> AAHHHHHHSSGLVPRGSHMANKAVNDFILAMNYDKKKLLTHQGESIENRFIKEGNQLPDEFVVIERKKRSLSTNTSDISVTATNDSRLYPGALLVVDETLLENNPTLLAVDRAPMTYSIDLPGLASSDSFLQVEDPSNSSVRGAVNDLLAKWHQDYGQVNNVPMQYEKITAHSMEQLKVKFGSDFEKTGNSLDIDFNSVHSGEKQIQIVNFKQIYYTVSVDAVKNPGDVFQDTVTVEDLKQRGISAERPLVYISSVAYGRQVYLKLETTSKSDEVEAAFEALIKGVKVAPQTEWKQILDNTEVKAVILGGDPSSGARVVTGKVDMVEDLIQEGSRFTADHPGLPISYTTSFLRDNVVATFQNSTDYVETKVTAYRNGDLLLDHSGAYVAQYYITWDELSYDHQGKEVLTPKAWDRNGQDLTAHFTTSIPLKGNVRNLSVKIRECTGLAWEWWRTVYEKTDLPLVRKRTISIWGTTLYPQVEDKVENAA

Gram-positive bacteria, including the common wound-infecting Staphylococcus aureus, the virulent food-borne pathogen Listeria monocytogenes, and Streptococcus pneumoniae that causes pneumonia, utilize cholesterol-dependent cytolysins (CDCs) to attack and kill mammalian and human cells. The bacteria produce and release CDCs as water-soluble monomers that attach to cholesterol-containing cell membranes, where they assemble into large, 200–500 Å cytolytic pores. X-ray structures of pneumolysin (PLY) from S. pneumoniae show that the soluble toxin monomers are roughly rod-shaped and consist of four domains (D1-D4). Sequence comparison suggests that all CDCs have the same domain structure and therefore insert into target membranes in essentially the same way.

We also deleted Ala146 and Arg147 (PLYΔ146/147) in the loop that would clash with the last β-strand of the central β-sheet. X-ray data were collected to 2.45 and 2.5 Å resolution from crystals of PLYD168A and PLYΔ146/147. Superposition of both structures on PLYWT showed no significant overall differences, although a detailed comparison indicated small changes in domain D2, helix bundle HB2 and in two of the D4 loops. Around the mutated residue in PLYD168A differences were restricted to sidechain orientations, while the deletion of two residues in PLYΔ146/147 caused significant conformational changes in the loop connecting helix α5 to strand β7 of the central β-sheet. In PLYΔ146/147, one loop connecting D1 to D3 is also slightly different (red arrows). (A) Ala146 and Arg147 in the loop that induces refolding of the last β-strand in the central D3 β-sheet into helix α13a in the late prepore and pore complex. Deletion of both residues renders the toxin inactive. Even though the structures of PLYD168A and PLYΔ146/147 were very similar to PLYWT, they displayed major differences in their membrane-binding and oligomerization behaviour. PLYΔ146/147 was not able to bind to the membranes at all and had no detectable hemolytic activity. The pivotal role of the loop that contains residues 145–147 connecting helix α5 of D1 to β7 of β-hairpin one is underlined by mutant PLYΔ146/147 that was completely inactive and did not even bind to liposomes.> GSHMASMSKDEVKREAKDTDGNPEIKGER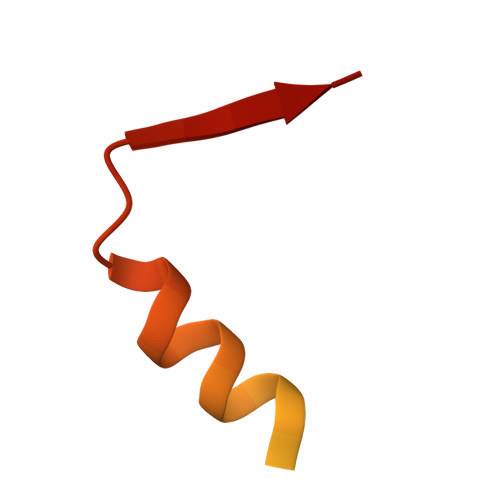RRLHSEIQSTSLANNIKKSTVIVKN>MAAALQTNIRTVKVPATFRAVSKQSLAPFRVRCAVASPGKKRYTITLLPGDGIGPEVVSIAKNVLQQAGSLEGVEFNFREMPIGGAALDLVGVPLPEETISAAKESDAVLLGAIGGYKWDNNEKHLRPEKGLLQIRAALKVFANLRPATVLPQLVDASTLKREVAEGVDLMVVRELTGGIYFGEPRGIKTNENGEEVGFNTEVYAAHEIDRIARVAFETARKRRGKLCSVDMANVLEASILWRKRVTALASEYPDVELSHMYVDNAAMQLVRDPKQFDTIVTNNIFGDILSDEASMITGSIGMLPSASLSDSGPGLFEPIHGSAPDIAGQDKANPLATILSAAMLLKYGLGEEKAAKRIEDAVLVALNNGFRTGDIYSAGTKLVGCKEMGEEVLKS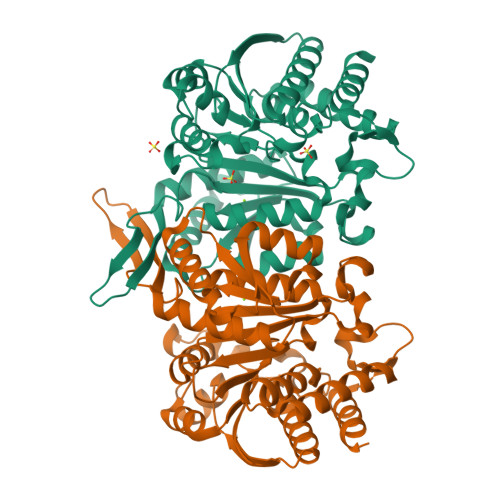VDSQVPASV[4x]> SNALSPVVNVDDMLRARWAEIQRGTGGRLGTCL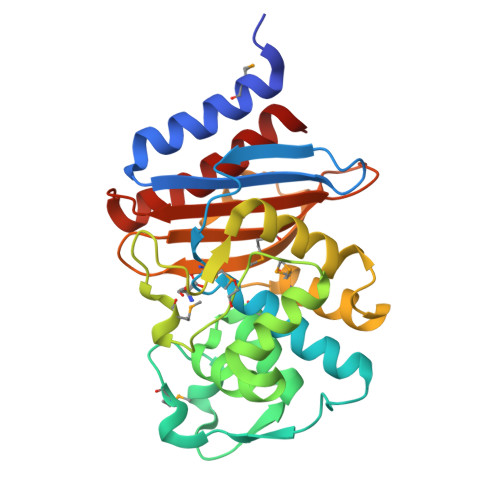LDSGSGWRIGQRENERFPMCSTFKFVLAAAVLQRVDKGELRLTQQIKIRASDMLEHAPVTERHVGGSLSVAELCQATMIHSDNPAANLLFPLIGDPPGLTRFLRGIGDTKTRSDRLEPAMNGFAPGEPRDTTTPAAMAATLRTLLLGDALQPASRKQLTAWMIDNRTGDDCLRAGLPRDWKIGDKTGSNGTDTRNDIAIIWPPGRAAPLLLTAYLNGATVDAAARDAALKAVAEAVRDLVG>[3x]ENKTRWLNPVATFADIATTYPNPQHGDTVMVTDDGENSGSVYRYENGQWNLTQKHNDLAIADVQNKIGILKTIAVNVKEFGTKGDGVTDDTVAIQNAINSIVSSLNNASGQGGIVYFPTGTY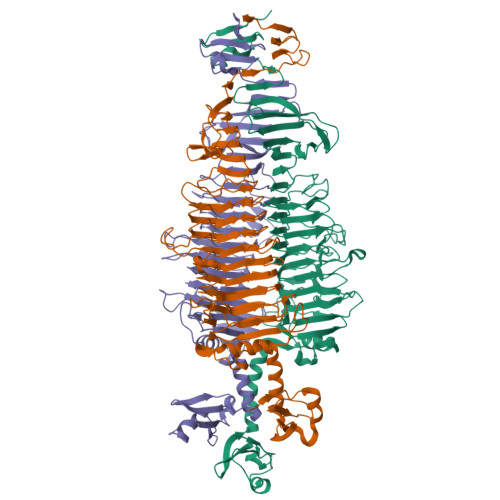KVTSKITINKSNIRLVGAGMSATCIKSTITNGNPVFEFVPSDTAQRLCFVGIEKMCIDGQNNDCIGVSLKKISLGRFLDFGVRYCANHGLYIEEVWDTNIIGLYNTDNGDLARNKHGVYIYNGTSDNSNRLLFIACHFEANNGSHVYFDSTGNRRRNGNNQFIGCKFHGKDPSALPGNNPNTPHMYLDGDVTYVMNCYFYQCNNDFIKVKGDRNKIIGCDFYNCTGYFVNLTGTSMLNVIDGCSGQYFGSGLAPFNNPTNENFFCSDFIGENRKLGWNRSYILDQGGRLALFQNVYRSGANFIQPKGTNASFGIQIADNTVDGVAFVGANASGTDNSNVTLTTLLNVTLDGIKPKVPITFTPVTASSTLNNSLFVDSADNKLKFKDNTGTVKIVTLT> KMTRPSSDLTAFREHFAKAKHIAIITGAGVSAESGVPTFRGPGGFWRKWQAQDLATPEAFSRDPSLVWEFYHYRREVMRSKMPNPAHLAIAECEARLGQQGRSVVIITQNIDELHHRAGSKHVYEIHGSLFKTRCMSCGEVKANHKSPICPALDGKGAPDPNTKEARIPVELLPRCERKSCNGLLRPHVVW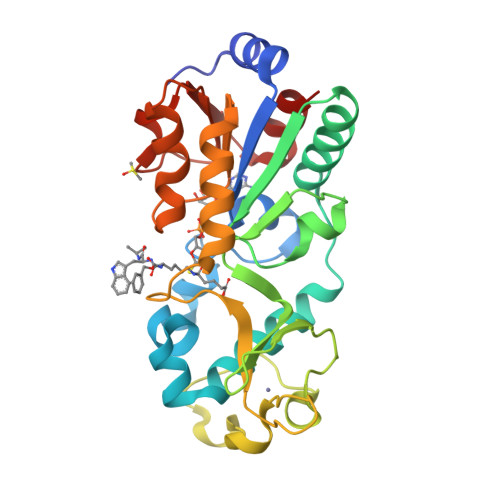FGETLDSDILTAVERELEKCDLCLVVGTSSIVYPAAMFAPQVASRGVPVAEFNMECTPATQRFKYHFEGPCGSTLPPALE3-({(2S)-3-[4-(2-aminoethyl)piperidin-1-yl]-2-[(naphthalen-2-ylsulfonyl)amino]-3-oxopropyl}oxy)benzenecarboximidamide 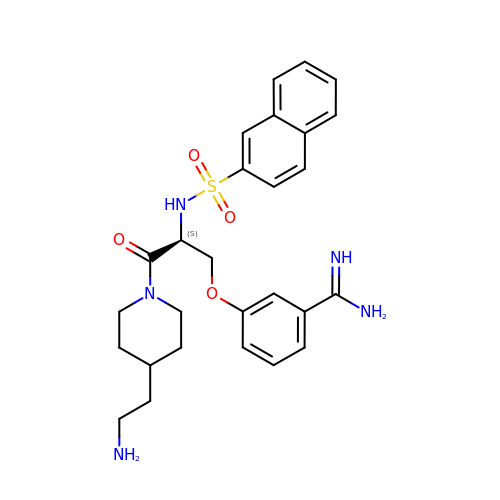| C27 H33 N5 O4 S | LNOODAVJDWKXFO-VWLOTQADSA-N premithramycin B | C53 H72 O24 | 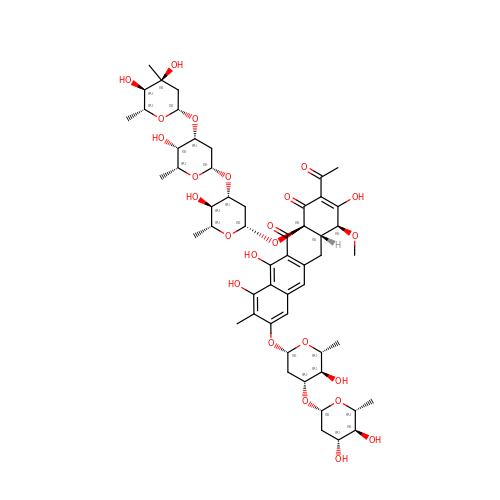HCTADUCAPFYREF-OFWAWROCSA-N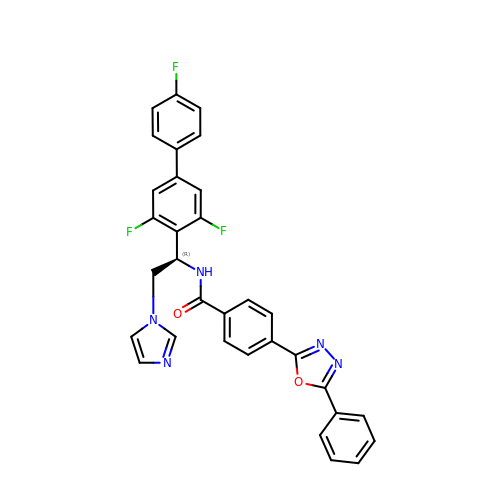N-[(1R)-2-(1H-imidazol-1-yl)-1-(3,4',5-trifluoro[1,1'-biphenyl]-4-yl)ethyl]-4-(5-phenyl-1,3,4-oxadiazol-2-yl)benzamide | C32 H22 F3 N5 O2 | VZHXYQRJRDRVFA-NDEPHWFRSA-N> KSCPNPGEIRNGQIDVPGGILFGATI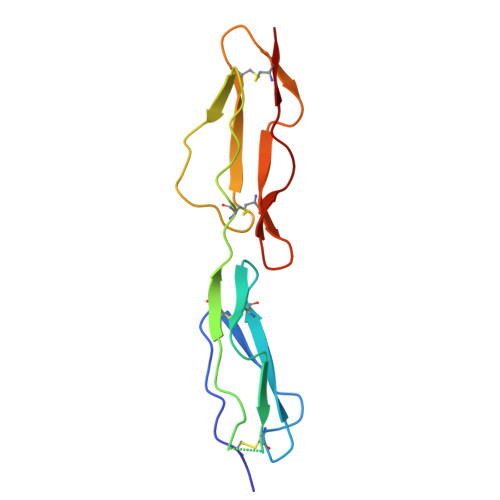SFSCNTGYKLFGSTSSFCLISGSSVQWSDPLPECREIYCPAPPQIDNGIIQGERDHYGYRQSVTYACNKGFTMIGEHSIYCTVNNDEGEWSGPPPECRG> MVVIANAHNEMIHDAVMDYYGKRMATCSSDKTIKIFEVEGETHKLIDTLTGHEGPVWRVDWAHPKFGTILASCSYDGKVMIWKEENGRWSQIAVHAVHSASVNSVQWAPHEYGPMLLVASSDGKVSVVEFKENGTTSPIIIDAHAIGVNSASWAPATIEEDGEHNGTKESRKFVTGGADNLVKIWKYNSDAQTYVLESTLEGHSDWVRDVAW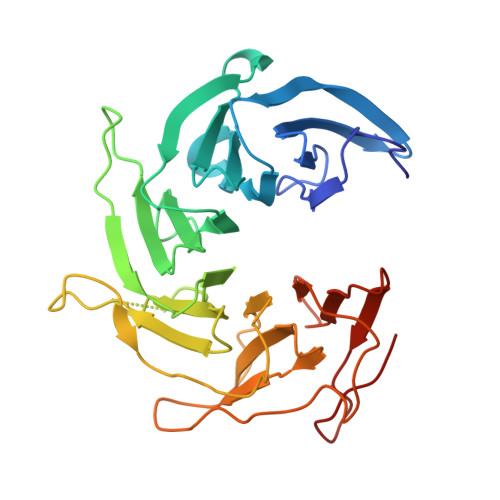SPTVLLRSYMASVSQDRTCIIWTQDNEQGPWKKTLLKEEKFPDVLWRASWSLSGNVLALSGGDNKVTLWKENLEGKWEPAGEVHQ>[12x]MSTLKIAPSILAADYANFASELARIEETDAEYVHIDIMDGQFVPNISFGADVVASMRKHSKLVFDCHLMVVDPERYVEAFAQAG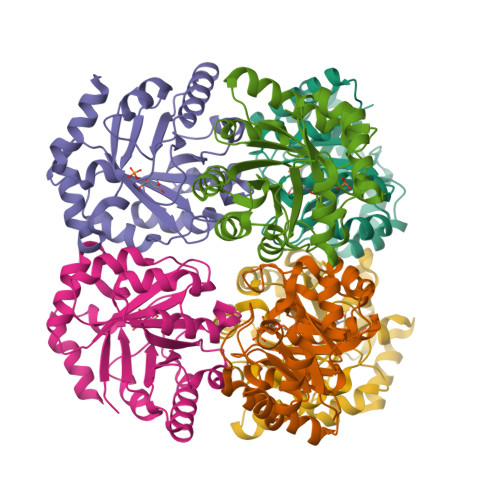ADIMTIHTESTRHIHGALQKIKAAGMKAGVVINPGTPATALEPLLDLVDQVLIMTVNPGFGGQAFIPECLEKVATVAKWRDEKGLSFDIEVDGGVDNKTIRACYEAGANVFVAGSYLFKASDLVSQVQTLRTALNV>MTHIYEPRLSRIAIDKLRPTQIAVGFREVELKRKEWRETRKKDGDDFLGNHIVPVVAGPKDRAYLIDHHHLVLALSKEGVEHVLTSEVAKFSHLGKDEFWSVMDHRNLIYPFDAQGLRRQSGDIPKNIHDLED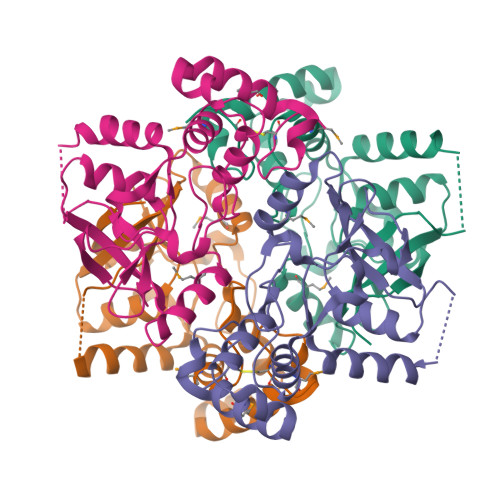DPFRSLAGALRMAGGYAKVIIPFSEFGWADFLRRRIDRDLLSDSFDDALAEAMKLAKSREARHLPGWCGVEE[6x]> AYAQWVIIIIHNVGSKDVKIKNLKPSWGKLHADGDKDTEVSASKYEGTVIKPDEKLQINACG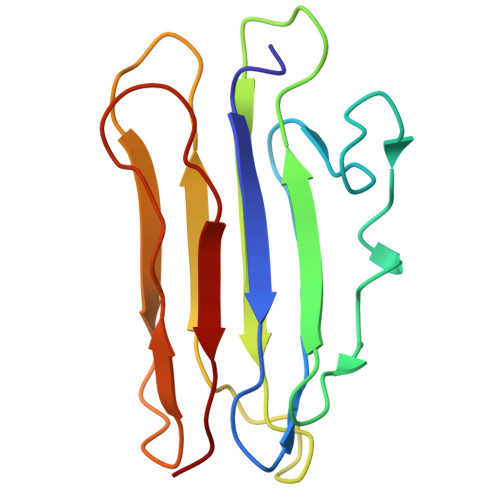RSDAAEGTTGTFDLVDPADGDKQVRHFYWDCPWGSKTNTWTVSGSNTKWMIEYSGQNLDSGALGTITVDTLKK> HHHHHHPEIVDTCSLASPASVCRTKHLHLRCSVDFTRRTLTGTAALTVQSQEDNLRSLVLDTKDLTIEKVVINGQEVKYALGERQSYKGSPMEISLPIALSKNQEIVIEISFETSPKSSALQWLTPEQTSGKEHPYLFSQCQAIHCRAILPCQDTPSVKLTYTAEVSVPKELVALMSAIRDGETPDPEDPSRKIYKFIQKVPIPCYLIALVVGALESRQIGPRTLVWSEKEQVEKSAYEFSETESMLKIAEDLGGPYVWGQYDLLVLPPSFPYGGMENPCLTFVTPTLLAGDKSLSNVIAHQISHSWTGNL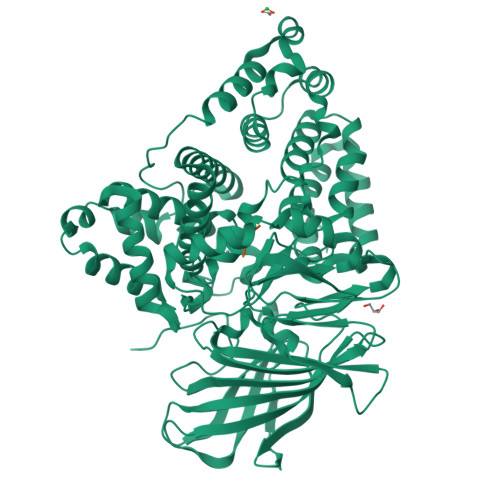VTNKTWDHFWLNEGHTVYLERHICGRLFGEKFRHFNALGGWGELQNSVKTFGETHPFTKLVVDLTDIDPDVAYSSVPYEKGFALLFYLEQLLGGPEIFLGFLKAYVEKFSYKSITTDDWKDFLYSYFKDKVDVLNQVDWNAWLYSPGLPPIKPNYDMTLTNACIALSQRWITAKEDDLNSFNATDLKDLSSHQLNEFLAQTLQRAPLPLGHIKRMQEVYNFNAINNSEIRFRWLRLCIQSKWEDAIPLALKMATEQGRMKFTRPLFKDLAAFDKSHDQAVRTYQEHKASMHPVTAMLVGKDLKVD;> RSR> MVNQVATDRFIQDLERVAQVRSEMSVCLNKLAETINKAELAGDSSSGKLSLERDIEDITIASKNLQQGVFRLLVLGDMKRGKSTFLNALIGENLLPSDVNPCTAVLTVLRYGPEKKVTIHFNDGKSPQQLDFQNFKYKYTIDPAEAKKLEQEKKQAFPDVDYAVVEYPLTLLQKGIEIVDSPGLNDTEARNELSLGYVNNCHAILFVMRASQPCTLGERRYLENYIKGRGLTVFFLVNAWDQVRESLIDPDDVEELQASENRLRQVFNANLAEYCTVEGQNIYDERVFELSSIQALRRRLKNPQADLDGTGFPKFMDSLNTFLTRERAIAELRQVRTLARLACNHTREAVARRIPLLEQDVNELKKRIDSVEPEFNKLTGIRDEFQKEIINTRDTQARTISESFRSYVLNLGNTFENDFLRYQPELNLFDFLSSGKREAFNAALQKAFEQYITDKSAAWTLTAEKDINAAFKELSRSASQYGASYNQITDQITEKLTGKDVKVHTTTTAEEDNSPGWAKWAMGLLSLSKGNLAGFALAGAGFDWKNILLNYFTVIGIGGIITAVTGILLGPIGFALLGLGVGFLQADQARRELVKTAKKELVKHLPQVAHEQSQVVYNAV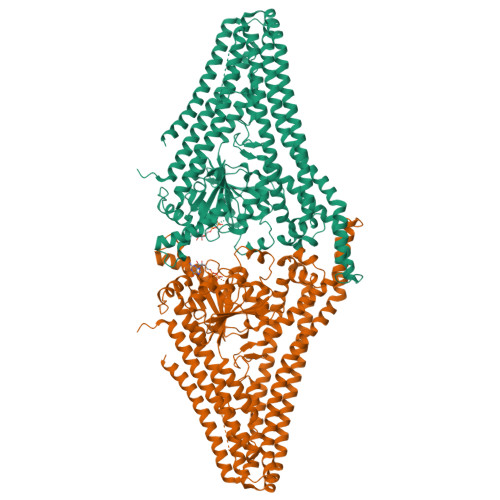KECFDSYEREVSKRINDDIVSRKSELDNLVKQKQTREINRESEFNRLKNLQEDVIAQLQKIEAAYSNLLAYYSHH> GPLGSMVSQETIKHVKDLIAENEIFVASKTYCPYC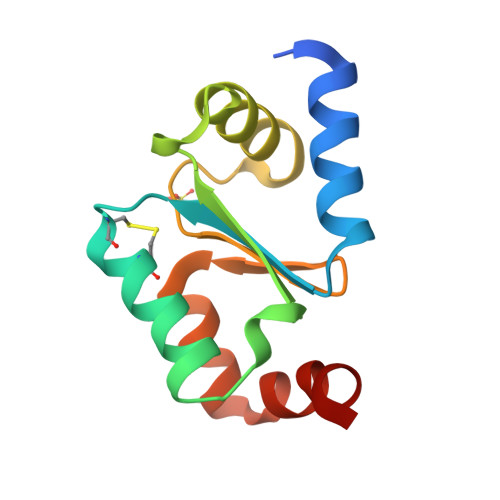HAALNTLFEKLKVPRSKVLVLQLNDMKEGADIQAALYEINGQRTVPNIYINGKHIGGNDDLQELRETGELEELLEPILAN>MTLIILEGPDCCFKSTVAAKLSKELKYPIIKGSSFELAKSGNEKLFEHFNKLADEDNVIIDRFVYSNLVYAKKFKDYSILTERQLRFIEDKIKAKAKVVYLHADPSVIKKRLRVRGDEYIEGKDIDSILELYREVMSNAGLHTY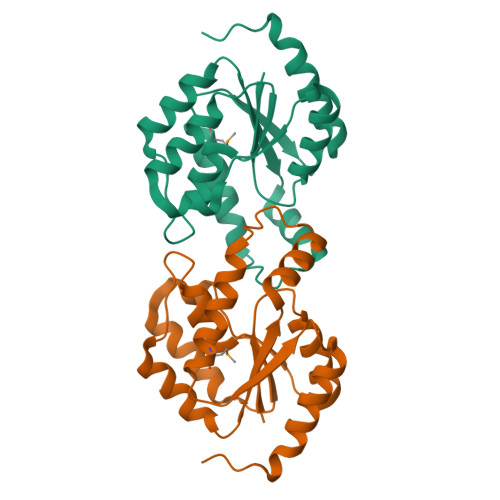SWDTGQWSSDEIAKDIIFLVELEHHHHHH[2x]>ELPQMTQQLNSDDMQEQLSATVKFRQILSREHRPPIDVVIQAGVVPRLVEFMRENQPEMLQLEAAWALTNIASGTSAQTKVVVDADAVPLFIQLLYTGSVEVKEQAIWALGNVAGDSTDYRDYVLQCNAMEPILGLFNSNKPSLIRTATWTLSNLCRGKKPQPDWSVVSQALPTLAKLIYSMDTETLVDACWAISYLSDGPQEAIQAVIDVRIPKRLVELLSHESTLVQTPALRAVGNIVTGNDLQTQVVINAGVLPALRLL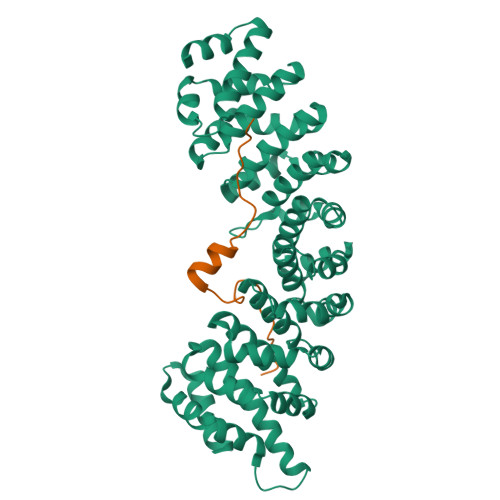LSSPKENIKKEACWTISNITAGNTEQIQAVIDANLIPPLVKLLEVAEYKTKKEACWAISNASSGGLQRPDIIRYLVSQGCIKPLCDLLEIADNRIIEVTLDALENILKMGEADKEARGLNINENADFIEKAGGMEKIFNCQQNENDKIYEKAYKIIETYF[2x];>GPLGSTNKRKREQISTDNEAKMQIQEEKSPKKKRKKRSSKANK[2x]> MFQCNVPLGMESGRIANEQISASSTYSDGRWTPQQSRLHGDDNGWTPNLDSNKEYLQVDLRFLTMLTAIATQGAISRETQNGYYVKSYKLEVSTNGEDWMV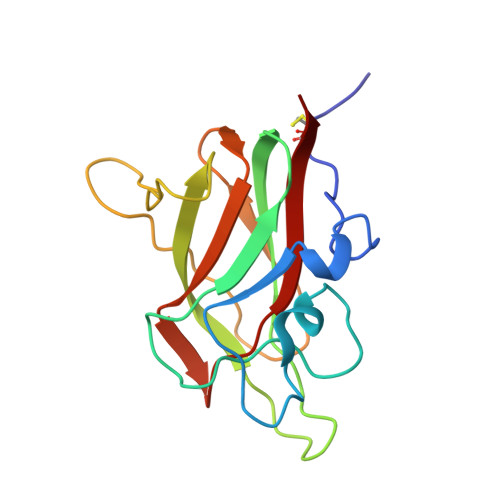YRHGKNHKVFQANNDATEVVLNKLHAPLLTRFVRIRPQTWHSGIALRLELFGCRV>[3x]GRRRVRAILPYTKVPDTDEISFLK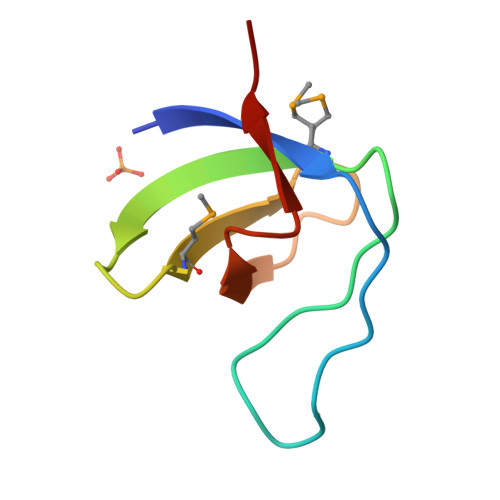GDMFIVHNELEDGWMWVTNLRTDEQGLIVEDLVEEVGR> GISPNVLNNMKSYMKHSNIRNIIINIMAHELSVINNHIKYINEL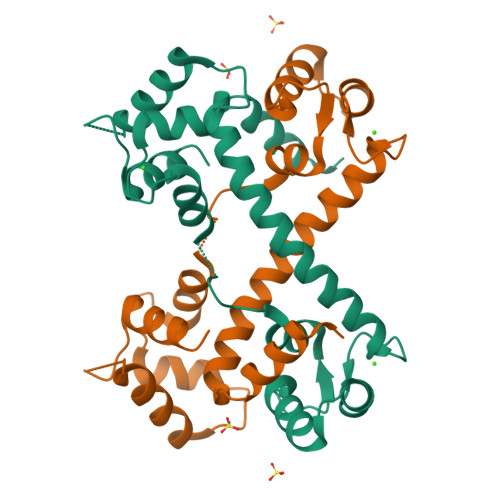FYKLDTNHNGSLSHREIYTVLASVGIKKWDINRILQALDINDRGNITYTEFMAGCYRWKNIESTFLKAAFNKIDKDEDGYISKSDIVSLVHDKVLDNNDIDNFFLSVHSIKKGIPREHIINKISFQEFKDYMLSTF>MKHQHQHQHQHQHQQPLNEEFRPEMLQGKKVIVTGASKGIGREMAYHLAKMGAHVVVTARSKETLQKVVSHCLELGAASAHYIAGTMEDMTFAEQFVAQAGKLMGGLDMLILNHITNTSLNLFHDDIHHVRKSMEVNFLSYVVLTVAALPMLKQSNGSIVVVSSLAGKVAYPMVAAYSASKFALDGFFSSIRKEYSVSRVNVSITLCVLGLIDTET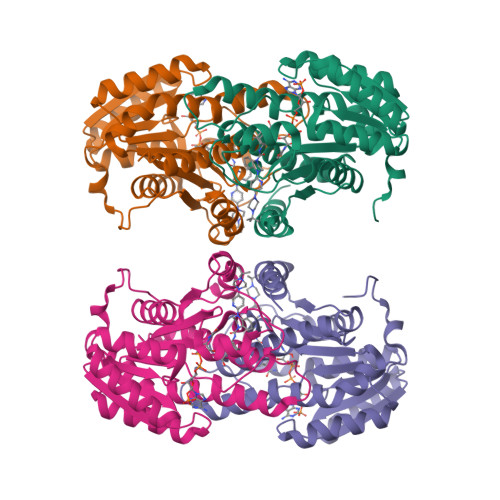AMKAVSGIVHMQAAPKEECALEIIKGGALRQEEVYYDSSLWTTLLIRNPSRKILEFLYSTSYNMDRFINK[4x]>MANTKYNKKFLLYLAGFVDGDGSIIAQINPNQSSKFKHRLRLTFYVTQKTQRRWFLDKLVDEIGVGYVRDSGSVSQYVLSEIKPLHNFLTQLQPFLKLKQKQANLVLKIIEQLPSAKESPDKFLEVCTWVDQIAALNDSKTRKTTSETVRAVLDSLSGKKKSSPAADWSHPQFEK[2x];>MANTKYNEEFLLYLAGFVDSDGSIIAQIKPRQSNKFKHQLSLTFAVTQKTQRRWFLDKLVDEIGVGYVYDSGSVSDYRLSEIKPLHNFLTQLQPFLKLKQKQANLVLKIIEQLPSAKESPDKFLEVCTWVDQI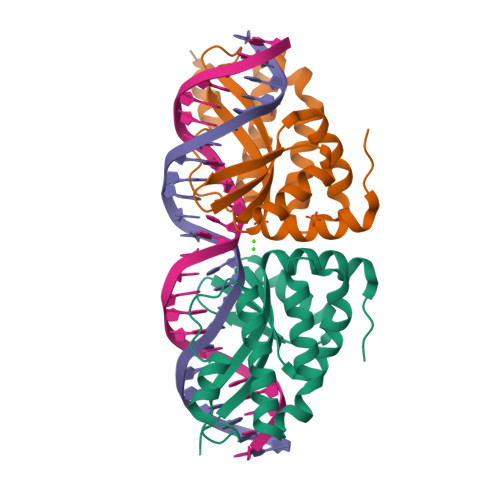AALNDSKTRKTTSETVRAVLDSLSEKKKSSPAADHHHHHH[2x]>GMVQTPSKPITLDEFLKLPETEPASEYIEGKIIQKPMPQGKHSAIQSECVSVINSVVKPQRIARAFLELRCTFGDHSTVPDISVFIWSRIPRE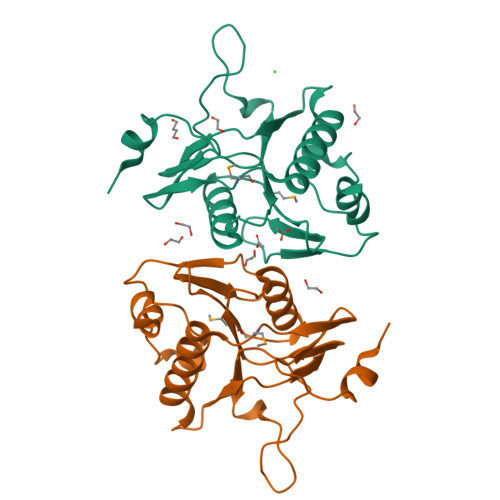ENGEIANIFLIAPDWTIEILSPDQSQTKVTKNILHCLKHGTQMGWLIDPDEQTVFVYRPQQETEVFDEPDALVPVPSFASELHLSIKDLFSWLL[2x]The Myxococcus xanthus FrzS protein transits from pole-to-pole within the cell, accumulating at the pole that defines the direction of movement in social (S) motility. The N-terminal receiver domain (RD), a 258-residue coiled-coil domain, and the extreme C-terminal tail of the protein are all required for the dynamic subcellular localization and S-motility activity of FrzS. Here we show using atomic-resolution crystallography and NMR that the FrzS receiver domain (RD) displays the conserved switch Tyr102 in an unusual conformation, lacks the conserved Asp phosphorylation site, and fails to bind Mg2+ or the phosphoryl analogue, Mg2+·BeF3. The crystal structures of the mutants suggested that the observed conformation of Tyr102 in the wild-type FrzS RD is not sufficient for function. These results support the model that FrzS contains a novel ‘pseudo-receiver domain’ whose function requires recognition of the RD output face but not Asp phosphorylation.

To explore the potential for intramolecular signalling, we determined the crystal structure of the FrzS RD in two crystal forms, a hexagonal form (P63) at 1.0 Å resolution and a tetragonal form (I4) at 1.9 Å. The hexagonal form was solved by molecular replacement using the first RD from the diguanylate cyclase PleD as the search model. The R/R-free values for all data to 1.0 Å resolution were 9.2/12.3%, below the average for structures at comparable resolution in the PDB. In the FrzS RD, the conserved Tyr102 adopted an ‘inward-facing’ rotamer. Remarkably, this conformation was distinct from those in either the inactive or active CheY. Furthermore, the conformation of Tyr102 is stabilized by hydrogen bonding of the hydroxyl group to His92 Nδ1, clearly visible in difference electron density in the high-resolution structure. In contrast to the CheY structure, we observed no conformational heterogeneity along the α4-β5-α5 face of the 1.0 Å FrzS RD structure, even at low contours of electron density below 0.25 σ. In the high-resolution hexagonal structure, a discrete minor population was modelled at 34% occupancy for the side-chain and backbone atoms of residues 55–62. This alternate conformation suggests a coordinated mode of motion, but this segment has not been implicated in dynamic rearrangements associated with RD signalling. The position of Tyr102 in FrzS is partially buried, suggesting that apo-FrzS does not prevent interactions along the α4-β5-α5 face by steric clashes with the switch tyrosine.

> GSHMSKKILIVESDTALSATLRSALEGRGFTVDETTDGKGSVEQIRRDRPDLVVLAVDLSAGQNGYLICGKLKKDDDLKNVPIVIIGNPDGFAQHRKLKAHADEYVAKPVDADQLVERAGALIGFPE N-methyl-N-{3-[({2-[(2-oxo-2,3-dihydro-1H-indol-5-yl)amino]-5-(trifluoromethyl)pyrimidin-4-yl}amino)methyl]pyridin-2-yl}methanesulfonamide 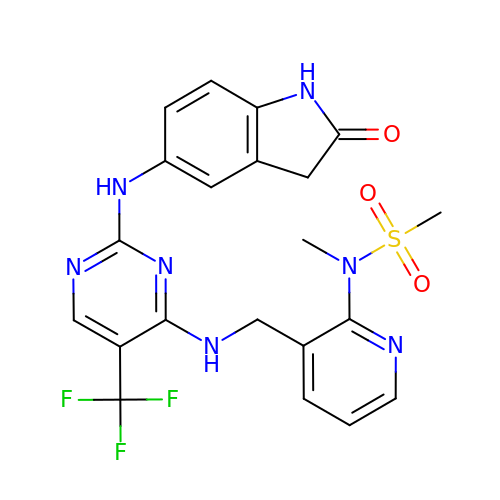| C21 H20 F3 N7 O3 S | MZDKLVOWGIOKTN-UHFFFAOYSA-N> MKVEELIIDGFKSYATRTVITDWDPQFNAITGLNGSGKSNILDAICFVLGIASMSTVRASSLQDLIYKRGQAGVTKASVTIVFDNTDKSNSPIGFTNSPQISVTRQVVLGGTSKYLINGHRAPQQSVLQLFQSVQLNINNPNFLIMQGKITKVLNMKPSEILSLIEEAAGTKMFEDRREKAERTMSKKETKLQENRTLLTEEIEPKLEKLRNEKRMFLEFQSTQTDLEKTERIVVSYEYYNIKHKHTSIRETLENGETRMKMLNEFVKKTSEEIDSLNEDVEEIKLQKEKELHKEGTISKLENKENGLLNEISRLKTSLSIKVENLNDTTEKSKALESEIASSSAKLIEKKSAYANTEKDYKMVQEQLSKQRDLYKRKEELVSTLTTGISSTGAADGGYNAQLAKAKTELNEVSLAIKKSSMKMELLKKELLTIEPKLKEATKDNELNVKHVKQCQETCDKLRARLVEYGFDPSRIKDLKQREDKLKSHYYQTCKNSEYLKRRVTNLEFNYTKPYPNFEASFVHGVVGQLFQIDNDNIRYATALQTCAGGRLFNVVVQDSQTATQLLERGRLRKRVTIIPLDKIYTRPISSQVLDLAKKIAPGKVELAINLIRFDESITKAMEFIFGNSLICEDPETAKKITFHPKIRARSITLQGDVYDPEGTLSGGSRNTSESLLVDIQKYNQIQKQIETIQADLNHVTEELQTQYATSQKTKTIQSDLNLSLHKLDLAKRNLDANPSSQIIARNEEILRDIGECENEIKTKQMSLKKCQEEVSTIEKDMKEYDSDKGSKLNELKKELKLLAKELEEQESESERKYDLFQNLELETEQLSSELDSNKTLLHNHLKSIESLKLENSDLEGKIRGVEDDLVTVQTELNEEKKRLMDIDDELNELETLIKKKQDEKKSSELELQKLVHDLNKYKSNTNNMEKIIEDLRQKHEFLEDFDLVRNIVKQNEGIDLDTYRERSKQLNEKFQELRKKVNPNIMNMIENVEKKEAALKTMIKTIEKDKMKIQETISKLNEYKRETLVKTWEKVTLDFGNIFADLLPNSFAKLVPCEGKDVTQGLEVKVKLGNIWKESLIELSGGQRSLIALSLIMALLQFRPAPMYILDEVDAALDLSHTQNIGHLIKTRFKGSQFIVVSLKEGMFANANRVFRTRFQDGTSVVSIM;> MSDSPLSKRQKRKSAQEPELSLDQGDAEEDSQVENRVNLSENTPEPDLPALEASYSKSYTPRKLVLSSGENRYAFSQPTNSTTTSLHVPNLQPPKTSSRGRDHKSYSQSPPRSPGRSPTRRLELLQLSPVKNSRVELQKIYDRHQSSSKQQSRLFINELVLENFKSYAGKQVVGPFHTSFSAVVGPNGSGKSNVIDSMLFVFGFRANKMRQDRLSDLIHKSEAFPSLQSCSVAVHFQYVIDESSGTSRIDEEKPGLIITRKAFKNNSSKYYINEKESSYTEVTKLLKNEGIDLDHKRFLILQGEVENIAQMKPKAEKESDDGLLEYLEDIIGTANYKPLIEERMGQIENLNEVCLEKENRFEIVDREKNSLESGKETALEFLEKEKQLTLLRSKLFQFKLLQSNSKLASTLEKISSSNKDLEDEKMKFQESLKKVDEIKAQRKEIKDRISSCSSKEKTLVLERRELEGTRVSLEERTKNLVSKMEKAEKTLKSTKHSISEAENMLEELRGQQTEHETEIKDLTQLLEKERSILDDIKLSLKDKTKNISAEIIRHEKELEPWDLQLQEKESQIQLAESELSLLEETQAKLKKNVETLEEKILAKKTHKQELQDLILDLKKKLNSLKDERSQGEKNFTSAHLKLKEMQKVLNAHRQRAMEARSSLSKAQNKSKVLTALSRLQKSGRINGFHGRLGDLGVIDDSFDVAISTACPRLDDVVVDTVECAQHCIDYLRKNKLGYARFILLDRLRQFNLQPISTPENVPRLFDLVKPKNPKFSNAFYSVLRDTLVAQNLKQANNVAYGKKRFRVVTVDGKLIDISGTMSGGGNHVAKGLMKLGTNQSDKVDDYTPEEVDKIERELSERENNFRVASDTVHEMEEELKKLRDHEPDLESQISKAEMEADSLASELTLAEQQVKEAEMAYVKAVSDKAQLNVVMKNLERLRGEYNDLQSETKTKKEKIKGLQDEIMKIGGIKLQMQNSKVESVCQKLDILVAKLKKVKSASKKSGGDVVKFQKLLQNSERDVELSSDELKVIEEQLKHTKLALAENDTNMNETLNLKVELKEQSEQLKEQMEDMEESINEFKSIEIEMKNKLEKLNSLLTYIKSEITQQEKGLNELSIRDVTHTLGMLDDNKMDSVKEDVKNNQELDQEYRSCETQDESEIKDAETSCDNYHPMNIDETSDEVSRGIPRLSEDELRELDVELIESKINELSYYVEETNVDIGVLEEYARRLAEFKRRKLDLNNAVQKRDEVKEQLGILKKKRFDEFMAGFNIISMTLKEMYQMITMGGNAELELVDSLDPFSEGVTFSVMPPKKSWRNITNLSGGEKTLSSLALVFALHKYKPTPLYVMDEIDAALDFRNVSIVANYIKERTKNAQFIVISLRNNMFELAQQLVGVYKRDNRTKSTTIKNIDILNRT;> MTTQLRYENNDDDERVEYNLFTNRSTMMANFEEWIKMATDNKINSRNSWNFALIDYFYDLDVLKDGENNINFQKASATLDGCIKIYSSRVDSVTTETGKLLSGLAQRKTNGASNGDDSNGGNGEGLGGDSDEANIEIDPLTGMPISNDPDVNNTRRRVYNRVLETTLVEFETIKMKELDQELIIDPLFKKALVDFDEGGAKSLLLNTLNIDNTARVIFDASIKDTQNVGQGKLQRKEEELIERDSLVDDENEPSQSLISTRNDSTVNDSVISAPSMEDEILSLGMDFIKFDQIAVCEISGSIEQLRNVVEDINQAKDFIENVNNRFDNFLTEEELQAAVPDNAEDDSDGFDMGMQQELCYPDENHDNTSHDEQDDDNVNSTTGSIFEKDLMAYFDENLNRNWRGREHWKVRNFKKANLVNKESDLLEETRTTIGDTTDKNTTDDKSMDTKKKHKQKKVLEIDFFKTDDSFEDKVFASKGRTKIDMPIKNRKNDTHYLLPDDFHFSTDRITRLFIKPGQKMSLFSHRKHTRGDVSSGLFEKSTVSANHSNNDIPTIADEHFWADNYERKEQEEKEKEQSKEVGDVVGGALDNPFEDDMDGVDFNQAFEGTDDNEEASVKLDLQDDEDHKFPIRENKVTYSRVSKKVDVRRLKKNVWRSINNLIQEHDSRKNREQSSNDSETHTEDESTKELKFSDIIQGISKMYSDDTLKDISTSFCFICLLHLANEHGLQITHTENYNDLIVNYEDLATTQAAS;> MSGFSLSEYLTKFQTTDRESYPRLQDPSRELNVIIDQLAVSPEQIDASPDSLEALIDLCHDFPHLTPKLQTQLSYLISSSLSNLSKDIKANLSSNVNFTEIGGLIPQWKRHLEEYGYLIQVLLTFLQDELHKVSSQSTNLNRSAKNSKNDSANVELFKRDCNQMENLLESITKLLEINLSKIFQTTPEKDLFIGLFTRPLFVLLEIEPVTKVSSLKMFIQRILAMCVKNHGQSSSIQSSLMTNLTYFLHLSVFNAELLKLLNDEYNYPQLTEDILKEISTRVFNAKDTTGPKAISNFLIKLSELSPGIMLRQMNLVITLLNNSSITLRCSVVEACGNIVAELAQDPQTMEHYKQQIAVLIELLEERFQDSNPYVRTKAIQGCSKICDLSSKFNKSKAKFTSLAVRSLQDRSSLVRRNSVKLLSKLLLKHPFKAIHGSQLRLSEWEEYLKGSESQLNSTLKKVESQETLNDTIERSLIEEEVEQDEGQCRTELEGSFNKSAELSRIENEVENINATNTSVLMKLKLMIVYYKDAISFIKEIHKSIELISNLLFSKNRNEVLESMDFLVLADAFDIELSEFGIKKMLHLVWMKGTNDEGTSISVHLIECYKQLFLTAPDSCNMQEKAAHIAKNLINLSIGASIADLASLEQLLGMMYEQKLIDQHVINILWAIYNSASKASMQKEQNVNNRDSEKGFSKEQIHGSIIILGMLSLADNEIALKGLESLLNIGLGAVGLKDLTLCRYSCLALERMVPKRSTIITKAINQELEDVAVKKLYAIIINYTKDNEYYPMCEQALSALFTISSKPDILATDLIREKTMMTFGKPEEEDSILSLEQSSRVVSLSQLLFIVGQVAIKTLVYLEKCEAEFKKRKIEAETRNGKVKNQGADVTNTTQDNGGDKELEMIGGTNEDDFTDAIQFVKENELLFGEKSILGKFCPIVEEIVSNSSRFSDPMLQRTATLCLEKLMCLSSKYCEKSLPLLITVMEKSPDPTIRSNAVLGLGDMAVCFNNLVDENTDYLYRRLHDENLMVQRTCLMTVTFLILAGQVKVKGQLGEMAKCLDNPDQGISDMCRLFFTELASKDNAIYNGFIDIFSNLSSDDLLGKESFKKIIKFLLTFIDKERHQKQLNEKLVGRLRKCETQKQWDDI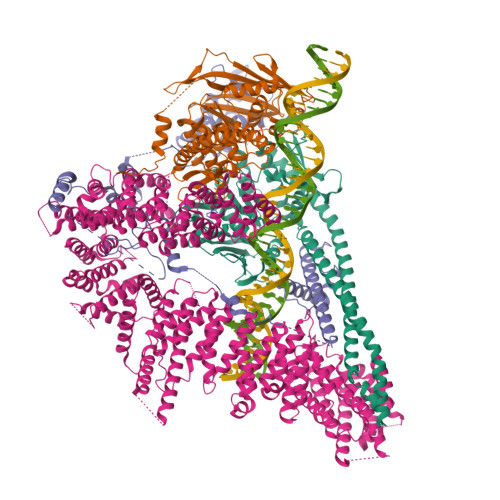AFVLNNLPYKNEDVTALLEQGFKVVSAKE>[2x]GMGISNIKQLYSKWKSLQPLKPEDLKRWNDKFKLEFNYNSNHLEGNTLTYGQTKLLLMFGETSGNASL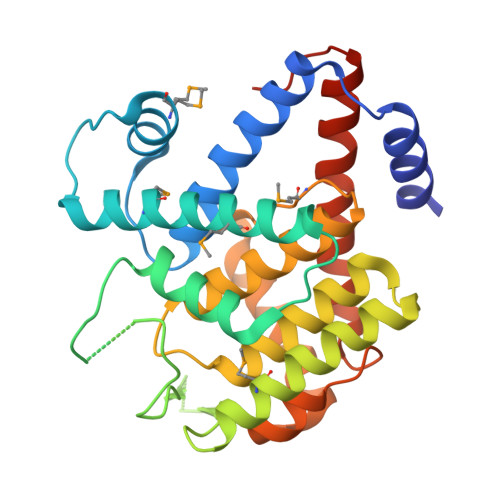KDYEEMKAHNVGLEMIKQEAQDKERPLTESFIRELNRTILVQDYWKNAKTPDGQDIRMQIKVGEYKSRPNSVLTATGEVFSYASPEETPAFMTSLVDWYNLEADKGILTPVELAALLHYRYIRIHPFEDGNGRIARLLVNFVLHRYGYPMIVIHSEDKSNYLNILHQCDVEAGLTPSDGANATLNDILPFVNYLSSCLIRSLTLAIKAAKGESIEEEGDFDKK>GEIEFIESSKDAGFPVINTPSKTKLEPSVFHQVFEGNKEPAVLRSGDPRLKANFEEAIFSKYIGNVNTHVDEYMLEAVDHYAGQLATLDISTEPMKLEDAVYGTEGLEALDLTTSAGYPYVALGIKKRDILSKKTKDLTKLKECMDKYGLNLPMVTYVKDELRSIEKVAKGKSRLIEASSLNDSVAMRQTFGNLYKTFHLNPGVVTGSAVGCDPDLFWSKIPVMLDGHLIAFDYSGYDASLSPVWFACLKMILEKLGYTHKETNYIDYLCNSHHLYRDKHYFVRGGMPSGCSGTSIFNSMINNIIIRTLMLKVYKGIDLDQFRMIAYGDDVIASYPWPIDASLLAEAGKGYGLIMTPADKGECFNEVTWTNVTFLKRYFRADEQYPFLVHPVMPMKDIHESIRWTKDPKNTQDHVRSLCLLAWHNGEHEYEEFIRKIRSVPVGRCLTLPAFSTLRRKWLDSFGSSSHHHHHH[4x]

The replication of positive-strand RNA viruses relies on virally encoded RNA-dependent RNA polymerases (RdRPs) that are capable of rapid and processive synthesis of the 7–14 kilobase viral genomes. To examine this in further detail and to validate the polymerase–RNA interactions seen in the initial poliovirus EC structures, we here present nine new coxsackievirus, rhinovirus, and poliovirus elongation complex structures at resolutions ranging from 2.1 to 2.9 Å. All the complexes feature an upstream RNA duplex that is pinched between the pinky finger and thumb domains such that the RNA exit channel is opened by ≈4 Å as compared to the polymerase alone structures. All of the complexes show the open conformation for the active site wherein the β-strands of motifs A and C are not hydrogen bonded together to fully form the RMM-fold that is commonly utilized by polymerase active sites.

Soaking the CV_r2 crystals with CTP results in cracking and a low resolution dataset (≈3.4 Å) that is not of sufficient quality to elucidate structural details, but soaking with 2′,3′-dideoxy-CTP (ddCTP) leads to a 2.7 Å resolution structure (CV_r2+1) reflecting one translocation event and a second ddCTP bound in the active site. This complex is stalled at the pre-catalysis state 2 of the catalytic cycle because the primer no longer has a reactive 3′-hydroxyl group following the first ddCTP incorporation event. The two polymerase molecules at opposite ends of the dumbbell remain essentially fixed and the translocation is accommodated by “peeling” nucleotides away from the end of the duplexes at the RNA-RNA junction so that they become disordered in solvent channels and are no longer resolved in the structure. There are minor perturbations at the end of the RNA helices as new non-canonical base stacking and hydrogen bonding interactions are formed by the nucleotides that have now been translocated into the junction regions. 3500 K composite SA-omit maps contoured at 1.5 σ are shown for the CV_r2 complexes where soaking with 2′,3′-ddCTP results in one incorporation and translocation event and the binding of a second ddCTP in the active site. In contrast, the coxsackievirus 3Dpol CV_r2 lattice accommodated one translocation event upon 2′,3′-ddCTP addition by keeping the two ECs within a dumbbell pair essentially fixed while unraveling the ends of the two RNA duplexes at the junction point.> SGATEACLPAGQRKSGMNINFYQYSLKDSSTYSNAAYMAYGYASKTKLGSVGGQTDISIDYNIPCVSSSGTFPCPQEDSYGNWGCKGMGACSNSQGIAYWSTDLFGFYTTPTNVTLEMTGYFLPPQTGSYTFKFATVDDSAILSVGGATAFNCCAQQQPPITSTNFTIDGIKPWGGSLPPNIEGTVYMYAGYYYPMKV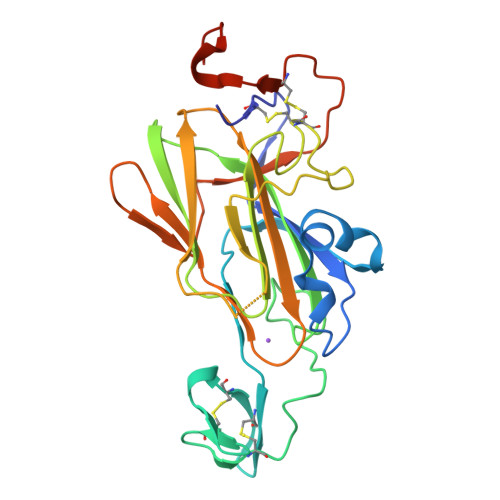VYSNAVSWGTLPISVTLPDGTTVSDDFEGYVYSFDDDLSQSNCTVPDPSNYLEVLFQGPHHHHHH>MEIERINEHTVKFYMSYGDIEDRGFDREEIWYNRERSEELFWEVMDEVHEEEEFAVEGPLWIQVQALDKGLEIIVTKAQLSKDGQKLELPIPEDKKQEPASEDLDALLDDFQKEEQAVNQEEKEQKLQFVLRFGDFEDVISLSKLNVNGSKTTLYSFENRYYLYVDFCNMTDEEVENQLSILLEYATESSISIHRLEEYGKLIISEHALETIKKHFAS[6x];>MMFGRFTERAQKVLALAQEEALRLGHNNIGTEHILLGLVREGEGIAAKALQALGLGSEKIQKEVESLIGRGQEMSQTIHYTPRAKKVIELSMDEARKLGHSYVGTEHILLGLIREGEGVAARVLNNLGVSLNKARQQVLQLLGSNETGSSAAGTNSNANTPTLDSLARDLTAIAKEDSLDPVIGRSKEIQRVIEVLSRRTKNNPVLIGEPGVGKTAIAEGLAQQIINNEVPEILRDKRVMTLDMGTVVAGTKYRGEFEDRLKKVMDEIRQAGNIILFIDALHTLIGAGGAEGAIDASNILKPSLARGELQCIGATTLDEYRKYIEKDAALERRFQPIQVDQPSVDESIQILQGLRDRYEAHHRVSITDDAIEAAVKLSDRYISDRFLPDKAIDLIDEAGSKVRLRSFTTPPNLKELEQKLDEVRKEKDAAVQSQEFEKAASLRDTEQRLREQVEDTKKSWKEKQGQENSEVTVDDIAMVVSSWTGVPVSKIAQTETDKLLNMENILHSRVIGQDEAVVAVAKAVRRARAGLKDPKRPIGSFIFLGPTGVGKTELARALAESIFGDEESMIRIDMSEYMEKHSTSRLVGSPPGYVGYDEGGQLTEKVRRKPYSVVLLDEIEKAHPD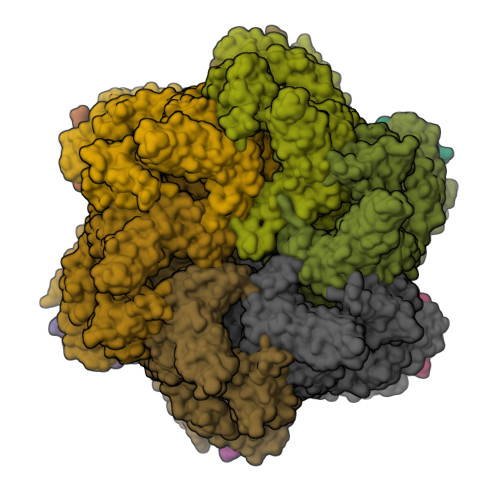VFNILLQVLEDGRLTDSKGRTVDFRNTILIMTSNVGASELKRNKYVGFNVQDETQNHKDMKDKVMGELKRAFRPEFINRIDEIIVFHSLEKKHLTEIVSLMSDQLTKRLKEQDLSIELTDAAKAKVAEEGVDLEYGARPLRRAIQKHVEDRLSEELLRGNIHKGQHIVLDVEDGEFVVKTTAKTN[6x]>[4x]MSNEIPKPVAPAPDILRCAYA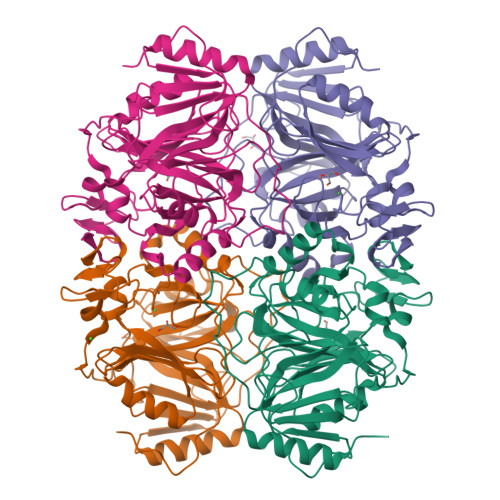ELVVTDLAKSRNFYVDVLGLHVSYEDENQIYLRSFEEFIHHNLVLTKGPVAALKAMAFRVRTPEDVDKAEAYYQELGCRTERRKDGFVKGIGDALRVEDPLGFPYEFFFETTHVERLHMRYDLYSAGELVRLDHFNQVTPDVPRGRKYLEDLGFRVTEDIQDDEGTTYAAWMHRKGTVHDTALTGGNGPRLHHVAFSTHEKHNIIQICDKMGALRISDRIERGPGRHGVSNAFYLYILDPDNHRIEIYTQDYYTGDPDNPTITWNVHDNQRRDWWGNPVVPSWYTEASKVLDLDGNVQEIILRTDDSELEVTIGADGFSFTRAGDEDGSYHGQASKGFKLGNQL> METGNKYIEKRAIDLSRERD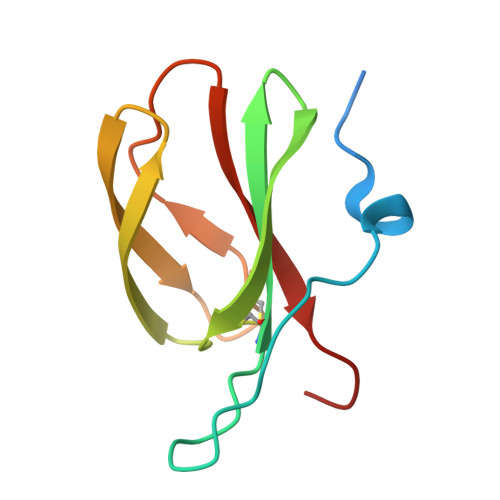PNFFDHPGIPVPECFWFMFKNNVRQDAGTCYSSWKMDMKVGPNWVHIKSDDNCNLSGDFPPGWIVLGKKRPGF>[4x]MRGSHHHHHHGSMKRVVITGLGIVSSIGNNQQE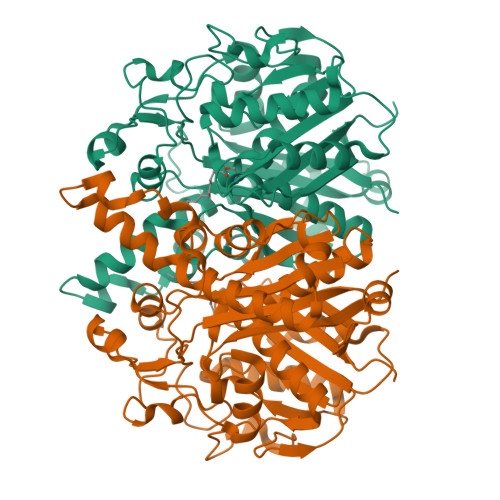VLASLREGRSGITFSQELKDSGMRSHVWGNVKLDTTGLIDRKVVRFMSDASIYAFLSMEQAIADAGLSPEAYQNNPRVGLIAGSGGGSPRFQVFGADAMRGPRGLKAVGPYVVTKAMASGVSACLATPFKIHGVNYSISSASATSAHCIGNAVEQIQLGKQDIVFAGGGEELCWEMACEFDAMGALSTKYNDTPEKASRTYDAHRDGFVIAGGGGMVVVEELEHALARGAHIYAEIVGYGATSDGADMVAPSGEGAVRCMKMAMHGVDTPIDYLNSHGTSTPVGDVKELAAIREVFGDKSPAISATKAMTGHSLGAAGVQEAIYSLLMLEHGFIAPSINIEELDEQAAGLNIVTETTDRELTTVMSNSFGFGGTNATLVMRKLKD> MTMPYYASAEQIMRDRSELARKGI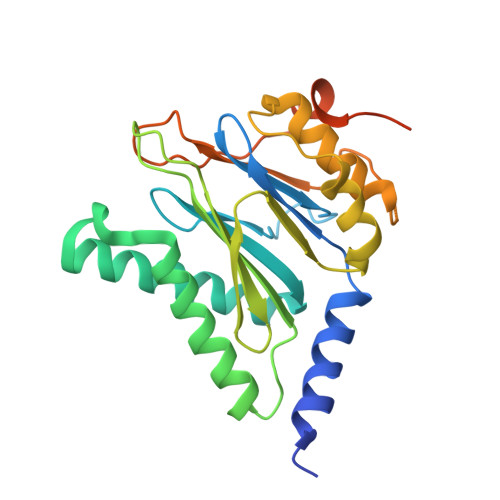ARGRSVVVLTFRDGVLFVAENPSTALHKVSELYDRLGFAAVGKYNEFENLRRAGIVHADMRGYSYDRRDVTGRSLANAYAQTLGTIFTEQPKPYEVEICVAEVGRVGSPKAPQLYRITYDGSIVDEQHFVVMGGTTEPIATAMRESYRADLDLEAAVGIAVNALRQGGAGEGEKRNVDVASLEVAVLDQSRPRRAFRRIAGTALEQLVPAEPAAASESAPEPKPDTETKPADTQD2-(2-methyl-1H-imidazol-1-yl)ethanol 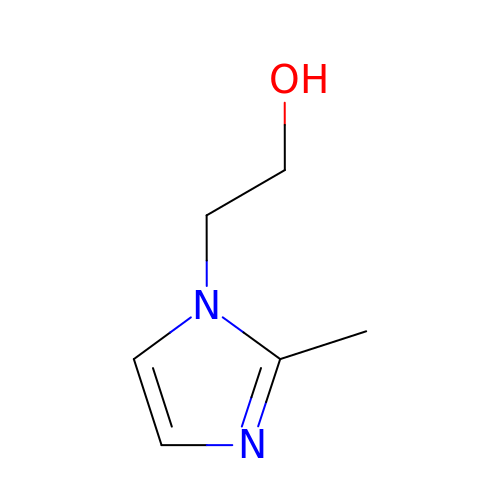| C6 H10 N2 O | JJWKKSUCSNDHNJ-UHFFFAOYSA-N> MTDQPDLFGLAPDAPRPIIPANLPEDWQEALLPEFSAPYFHELTDFLRQERKEYTIYPPAPDVFNALRYTPLGEVKVLILGQDPYHGPNQAHGLSFSVRPGVRVPPSLRNIYKELTEDIPGFVAPKHGYLRSWAEQGVLLLNAVLTVRAGQANSHQGKGWEHFTDAVIKAVNAKEERVVFILWGSYARKKKKLITGKNHVVIESGHPSPLSEQYFFGTRPFSKTNEALEKAGRGPVEWQLPAT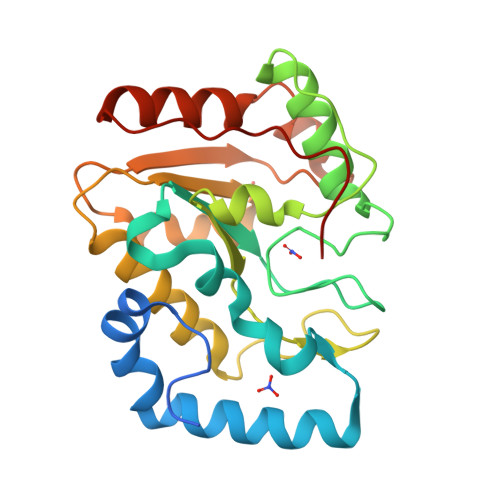VTEE(2S)-2-[2-(4-chlorophenyl)-5,6-difluoro-1H-benzimidazol-1-yl]-2-cyclohexyl-N-(2-fluorophenyl)acetamide 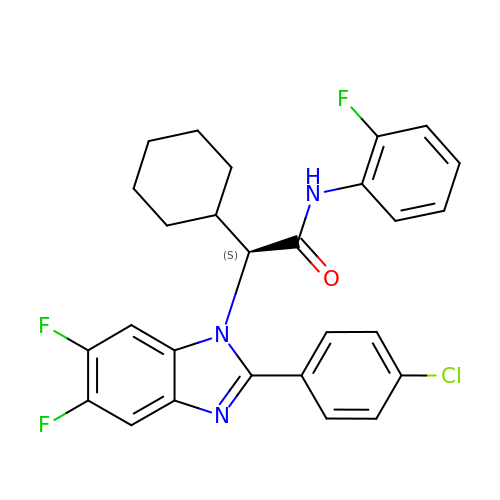| C27 H23 Cl F3 N3 O | JBLFHKBJHMUDCM-VWLOTQADSA-N> LYPEEILDTHWELWKKTHRKQYNNKVDEISRRLIWEKNLKYISIHNLEASLGVHTYELAMNHLGDMTS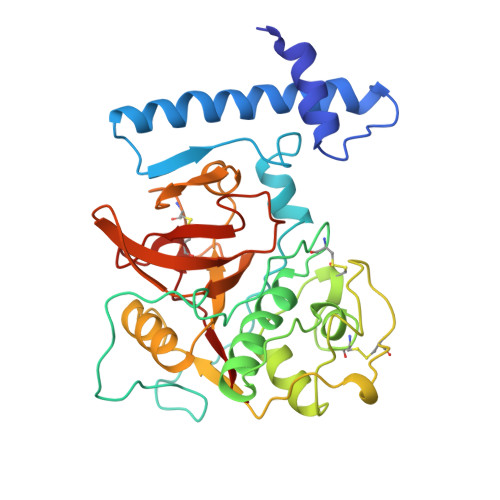EEVVQKMTGLKVPLSHSRSNDTLYIPEWEGRAPDSVDYRKKGYVTPVKNQGQCGSCWAFSSVGALEGQLKKKTGKLLNLSPQNLVDCVSENDGCGGGYMTNAFQYVQKNRGIDSEDAYPYVGQEESCMYNPTGKAAKCRGYREIPEGNEKALKRAVARVGPVSVAIDASLTSFQFYSKGVYYDESCNSDNLNHAVLAVGYGIQKGNKHWIIKNSWGENWGNKGYILMARNKNNACGIANLASFPKM>[2x]TAPSQVLKIRRPDDWHLHLRDGDMLKTVVPYTSEIYGRAIVMPNLAPPVTTVEAAVAYRQRILDAVPAGHDFTPLMTCYLTDSLDPNELERGFNEGVFTAAKLYPANAGTNSSHGVTSVDAIMPVLERMEKIGMPLLVHGEVTHADIDIFDREARFIESVMEPLRQRLTALKVVFEHITTKDAADYVRDGNERLAATITP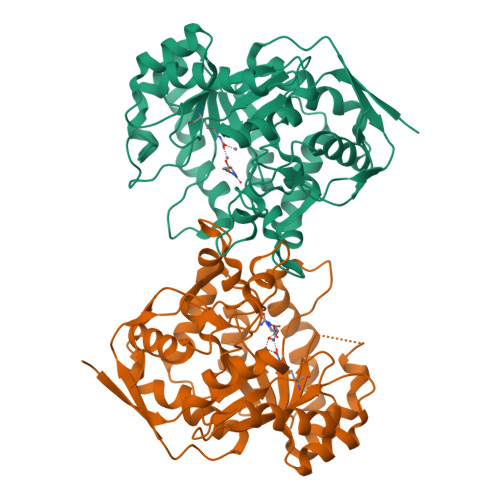QHLMFNRNHMLVGGVRPHLYCLPILKRNIHQQALRELVASGFNRVFLGTDSAPHARHRKESSCGCAGCFNAPTALGSYATVFEEMNALQHFEAFCSVNGPQFYGLPVNDTFIELVREEQQVAESIALTDDTLVPFLAGETVRWSVKQ>[2x]LHLDQTPSRQPIPSEGLQLHLPQVLADAVSRLVLGKFGDLTDNFSSPHARRKVLAGVVMTTGTDVKDAKVISVSTGTKCINGEYMSDRGLALNDCHAEIISRRSLLRFLYTQ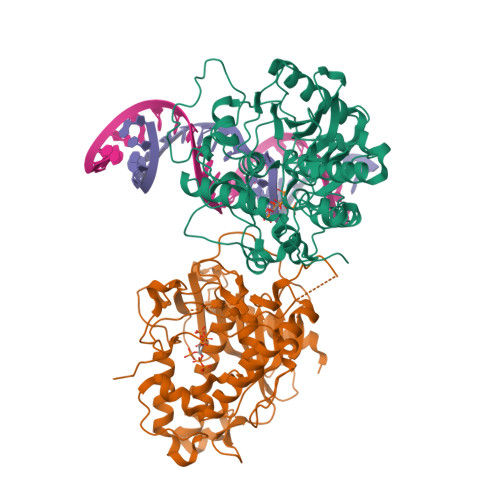LELYLNNKDDQKRSIFQKSERGGFRLKENVQFHLYISTSPCGDARIFSPHEPILEEPADRHPNRKARGQLRTKIESGEGTIPVRSNASIQTWDGVLQGERLLTMSCSDKIARWNVVGIQGSLLSIFVEPIYFSSIILGSLYHGDHLSRAMYQRISNIEDLPPLYTLNKPLLSGISNAEARQPGKAPNFSVNWTVGDSAIEVINATTGKDELGRASRLCKHALYCRWMRVHGKVPSHLLRSKITKPNVYHESKLAAKEYQAAKARLFTAFIKAGLGAWVEKPTEQDQFSLTP> GCGGCGUUGCGUCCGAAAGUCUAAACAGACACG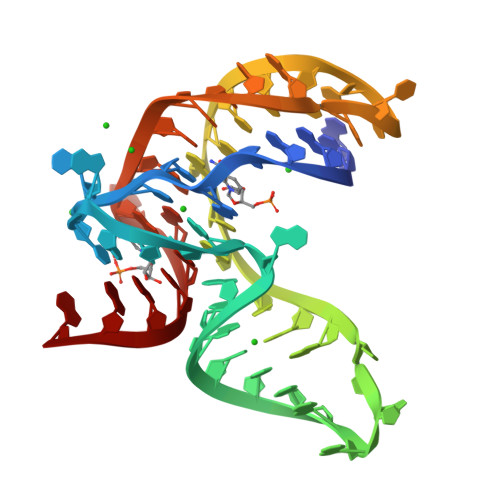GCCGCUUAAAAACAAAAGGAGA>GGSGPLKPEEHEDILNKLLDPELAQSERTEALQQLRVNYGSFVSEYNDLTKSHEKLEKVRKQLEAEKM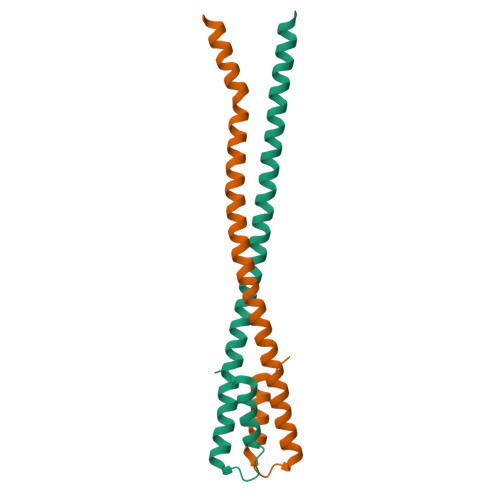ELQSALEEAEASLEHEEGKILRAQLEFNQIKAE[8x]>GSHMTNTGGRKPDEGERYRAILETAARLICDRGYEGTSMQEIAAACRMTKAGLYHHIQNKEQLLFAIMNYGMDLFEEQVLSRVQDIANPVERLRACMRHNILLVTRGWSKEVIIILHEHATLTGETRAFIDARKKKYVDFLEEAFSQASQQGLIRPVDPTVGAFSFLGMVLWIYKWFKPDGRLTDEQ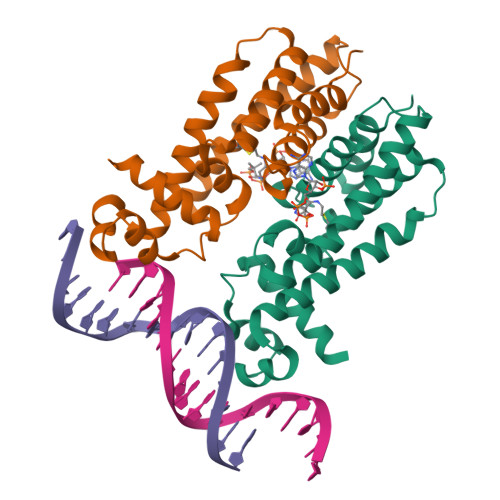IADGMVGMLFPPFAAAGDTAGQAGPSPLRMVPSVSATGTDSEDA[4x]methyl (2R)-2-[(4S)-6-(4-chlorophenyl)-8-methoxy-1-methyl-4H-[1,2,4]triazolo[4,3-a][1,4]benzodiazepin-4-yl]butanoate 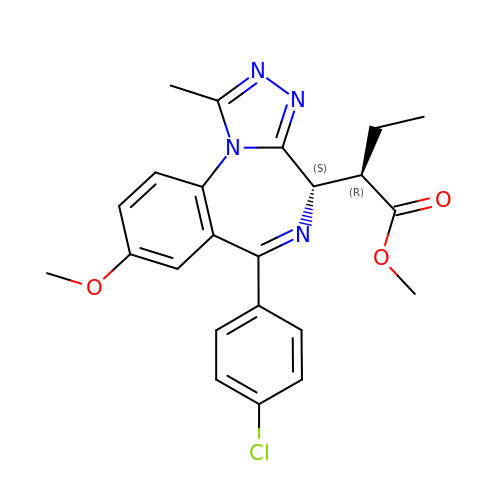| C23 H23 Cl N4 O3 | WGMDCNPABCIZCD-UTKZUKDTSA-N>AMGSMLSIEEERFLDAAEYGNIPVVRKMLEECHSLNVNCVDYMGQNALQLAVANEHLEITELLLKKENLSRVGDALLLAISKGYVRIVEAILNHPAFAEGKRLATSPSQSELQQDDFYAYDEDGTRFSHDVTPIILAAHCQEYEIVHTLLRKGARIERPHDYFCKCTECSQKQKHDSFSHSRSRINAYKGLASPAYLSLSSEDPVMTALELSNELAVLANIEKEFKNDYRKLSMQCKDFVVGLLDLCRNTEEVEAILNGDAETRQPGDFGRPNLSRLKLAIKYEVKKFVAHPNCQQQLLSIWYENLSGLRQQTMAVKFLVVLAVAIGLPFLALIYWCAPCSKMGKILRGPFMKFVAHAASFTIFLGLLVMNAADRFEGTKLLPNETSTDNARQLFRMKTSCFSWMEMLIISWVIGMIWAECKEIWTQGPKEYLFELWNMLDFGMLAIFAASFIARFMAFWHASKAQSIIDANDTLKDLTKVTLGDNVKYYNLARIKWDPTDPQIISEGLYAIAVVLSFSRIAYILPANESFGPLQISLGRTVKDIFKFMVIFIMVFVAFMIGMFNLYSYYIGAKQNEAFTTVEESFKTLFWAIFGLSEVKSVVINYNHKFIENIGYVLYGVYNVTMVIVLLNMLIAMINSSFQEIEDDADVEWKFARAKLWFSYFEEGRTLPVPFNLVPSPKSLLYLLLKFKKWMCEL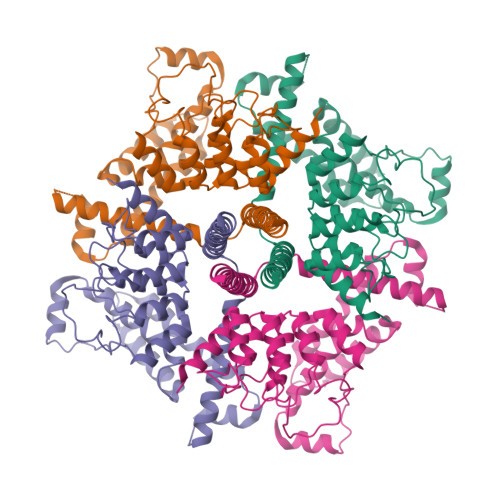IQGQKQGFQEDAEMNKRNEEKKFGISGSHEDLSKFSLDKNQLAHNKQSSTRSSEDYHLNSFSNPPRQYQKIMKRLIKRYVLQAQIDKESDEVNEGELKEIKQDISSLRYELLEEKSQNTEDLAELIRKLGERLSLEPKLEESRR[4x]> MNKHSGIDFKQLNFLTKLNENHSGELWKGRWQGNDIVVKVLKVRDWSTRKSRDFNEECPRLRIFSHPNVLPVLGACQSPPAPHPTLITHWMPYGSLYNVLHEGTNFVVDQSQAVKFALDMARGMAFLHTLEPLIPRHALNSRSVMIDEDMTARISMADVKFSFQSPGRMYAPAWVAPEALQKKPEDTNRRSADMWSFAVLLWELVTREVPFADLSNMEIGMKVALEGLRPTIPPGISPHVSKLMKICMNEDPA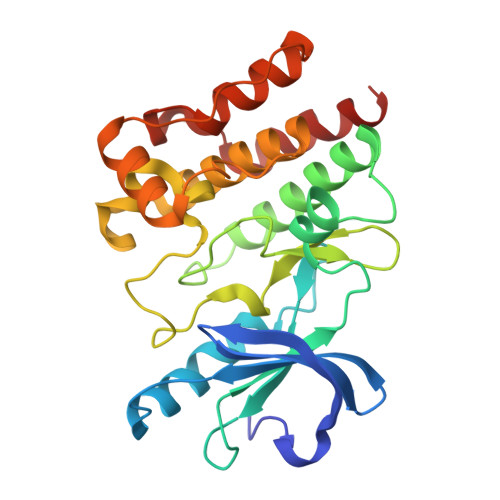KRPKFDMIVPILEKMQDK>PAPHGGILQDLIARDALKKNELLSEAQSSDILVWNLTPRQLCDIELILNGGFSPLTGFLNENDYSSVVTDSRLADGTLWTIPITLDVDEAFANQIKPDTRIALFQDDEIPIAILTVQDVYKPNKTIEAEKVFRGDPEHPAISYLFNVAGDYYVGGSLEAIQLPQHYDYPGLRKTPAQLRLEFQSRQWDRVVAFQTRNPMHRAHRELTVRAAREANAKVLIHPVVGLTKPGDIDHHTRVRVYQEIIKRYPNGIAFLSLLPLAMRMSGDREAVWHAIIRKNYGASHFIVGRDHAGPGKNSKGVDFYGPYDAQELVESYKHELDIEVVPFRMVTYLPDEDRYA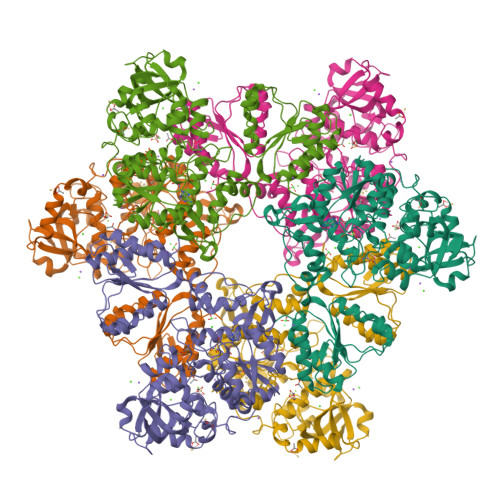PIDQIDTTKTRTLNISGTELRRRLRVGGEIPEWFSYPEVVKILRESNPPRPKQGFSIVLGNSLTVSREQLSIALLSTFLQFGGGRYYKIFEHNNKTELLSLIQDFIGSGSGLIIPNQWEDDKDSVVGKQNVYLLDTSSSADIQLESADEPISHIVQKVVLFLEDNGFFVF[2x]> MSALYFQNLPSRPANKENYTRLLLKHINPNNKYAINPSLPLPHNKLQISSQPLMLLDDQMGLLEVSISRSSKMTNQAFLTFVTQEEADRFLEKYTTTALKVQGRKVRMGKARTNSLLGLSIEMQKKKGNDETYNLDIKKVLKARKLKRKLRSDDICAKKFRLKRQIRRLKHKLRSRKVEEAEIDRIVKEFETRRLENMKSQQENLKQSQKPLKRAKVSNTMENPPNKVLLIQNLPSGTTEQLLSQILGNEALVEIRLVSVRNLAFVEYETVADATKIKNQLGSTY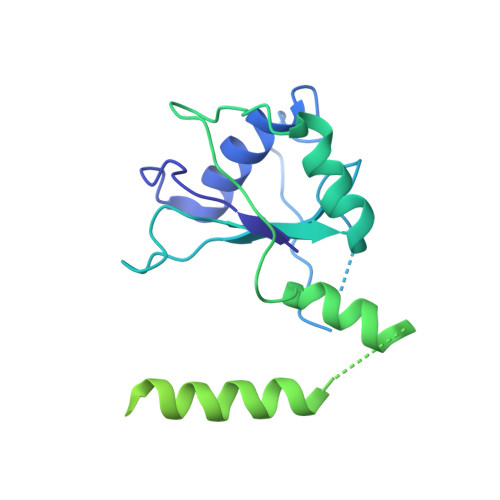KLQNNDVTIGFAK> SQNQERLCAFKDPYQQDLGIGESRISHENGTILCSKGSTCYGLWEKSKGDINLVKQGCWSHI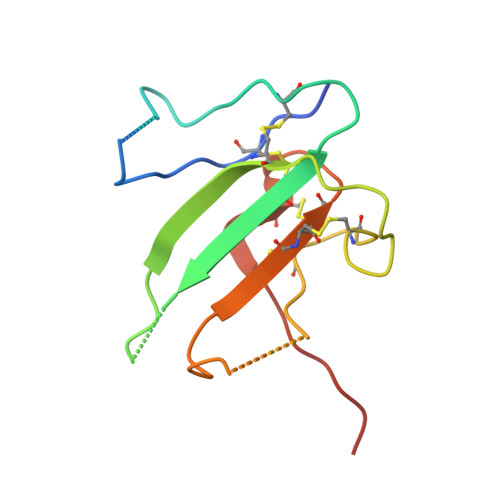GDPQECHYEECVVTTTPPSIQNGTYRFCCCSTDLCNVNFTENFPPPDTT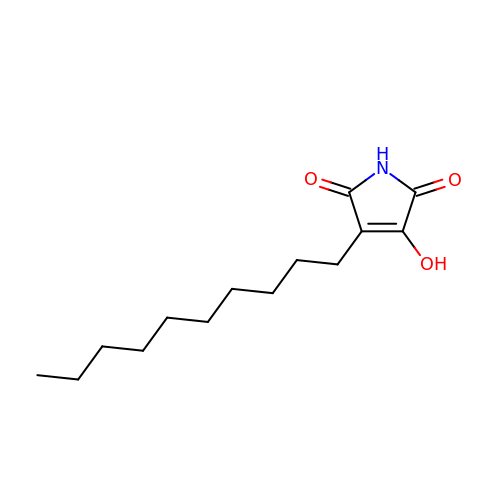3-DECYL-2,5-DIOXO-4-HYDROXY-3-PYRROLINE | C14 H23 N O3 | LXIDJQZEXUQBGG-UHFFFAOYSA-N>[2x]MPVAGSELQYLGQIQHILRCGVRKDDRTGTGTLSVFGMQARYSLRDEFPLLTTKRVFWKGVLEELLWFIKGSTNAKELSSKGVKIWDANGSRDFLDSLGFSTREEGDLGPVYGFQWRHFGAEYRDMESDYSGQGVDQLQRVIDTIKTNPDDRRIIMCAWNPRDLPLMALPPCHA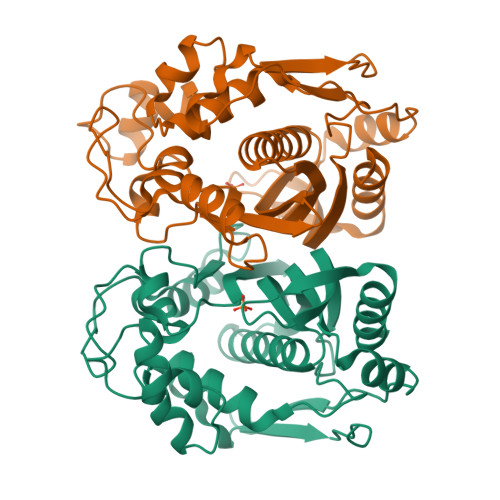LCQFYVVNSELSCQLYQRSGDMGLGVPFNIASYALLTYMIAHITGLKPGDFIHTLGDAHIYLNHIEPLKIQLQREPRPFPKLRILRKVEKIDDFKAEDFQIEGYNPHPTIKMEMAV>[36x]MSFFHGVTVTNVDIGARTIALPASSVIGLCDVFTPGAQASAKPNVPVLLTSKKDAAAAFGIGSSIYLACEAIYNRAQAVIVAVGVETAETPEAQASAVIGGISAAGERTGLQALLDGKSRF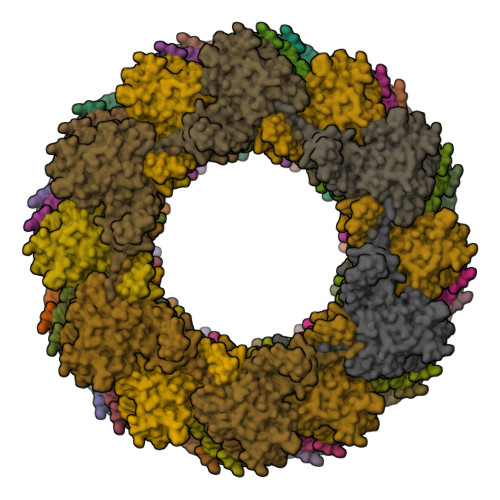NAQPRLLVAPGHSAQQAVATAMDGLAEKLRAIAILDGPNSTDEAAVAYAKNFGSKRLFMVDPGVQVWDSATNAARNAPASAYAAGLFAWTDAEYGFWSSPSNKEIKGVTGTSRPVEFLDGDETCRANLLNNANIATIIRDDGYRLWGNRTLSSDSKWAFVTRVRTMDLVMDAILAGHKWAVDRGITKTYVKDVTEGLRAFMRDLKNQGAVINFEVYADPDLNSASQLAQGKVYWNIRFTDVPPAENPNFRVEVTDQWLTEVLDVA> VFHKIRNEDLIFNESLGQGTFTKIFKGVRREVGDYGQLHETEVLLKVLDK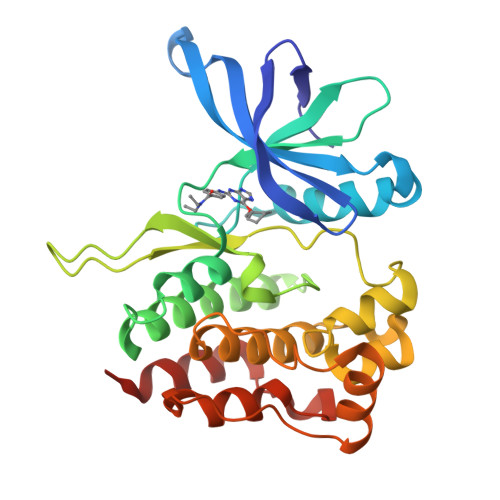AHRNYSESFFEAASMMSKLSHKHLVLNYGVCVCGDENILVQEFVKFGSLDTYLKKNKNCINILWKLEVAKQLAAAMHFLEENTLIHGNVCAKNILLIREEDRKTGNPPFIKLSDPGISITVLPKDILQERIPWVPPECIENPKNLNLATDKWSFGTTLWEICSGGDKPLSALDSQRKLQFYEDRHQLPAPKAAELANLINNCMDYEPDHRPSFRAIIRDLNSLFTPD phytanoyl-CoA | C41 H74 N7 O17 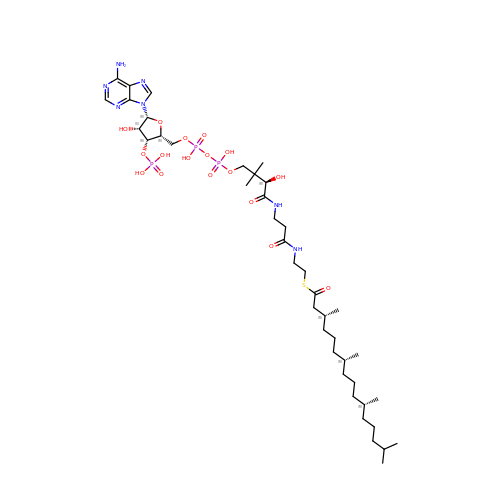P3 S | NRJQGHHZMSOUEN-SOYJUKJHSA-N> MGNCNKPPKRPPNTQTSSNQPSAEFRRTAPPSLYGRYNCKCCWFADTNLITCNDHYLCLRCHQTMLRNSELCHICWKPLP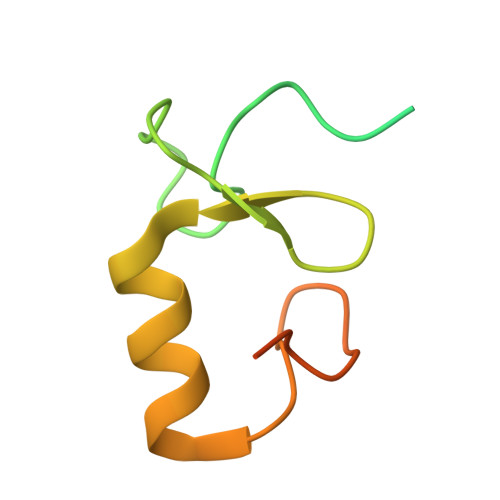TSITVPVEPSAPPP> GAMEATPTPADLFSEDYLVDTLDGLTVDDQQAVLASLSFSKFLKHAKVRDWCAQAKIQPSMPALRMAYNYFLFSKVGEFIGSEDVCNFFVDRVFGGVRLLDVASVYAACSQMNAHQRHHICCLVERATSSQSLNPVWDALRDGIISSSKFHWAVKQQNTSKKIFSPWPITNNHFVAGPLAFGLRCEEVVKTLLATLLHPDETNCLDYGFMQSPQNGIFGVSLDFAANVKTDTEGRLQFDPNCKVYSIKCRFKYTFAKMECDPIYAAYQRLYEAPGKLALKDFFYSISKPAVEYVGLGKLPSESDYLVAYDQEWEACPRKKRKLTPLHNLIRECILHNSTTESDVYVLTDPQDTRGQISIKARFKANLFVNVRHSYFYQVLLQSSIVEEYIGLDSGIPRLGSPKYYIATGFFRKRGYQDPVNCTIGGDALDPHVEIPTLLIVTPVYFPRGAKHRLLHQAANFWSRSAKDTFPYIKWDFSYLSANVPHSP

Transition to the lytic phase coincides with the rapid degradation of ∼80% of all host mRNA transcripts in a process termed host shutoff (HSO) that is thought to promote immune evasion and enable viral co-option of the host replicative machinery. In the γ-herpesviridiae, HSO is initiated by the bifunctional alkaline exonuclease SOX that has been shown to possess exonucleolytic DNase and RNase activities. Owing to the presence of a PD-(D/E)XK sequence spanning two of seven conserved motifs shown to be essential for DNA turnover, KSHV SOX has been classified as a member of the type II restriction endonuclease-like superfamily confirmed by the crystal structures of the the related Epstein–Barr virus alkaline exonuclease BGLF5 (3) and apo form. More recent in vivo studies, however, indicate that SOX-mediated HSO is instead initiated by endonucleolytic ‘nicking’ of target transcripts followed by exonucleolytic degradation by the co-opted host scavenger exoribonuclease Xrn1 reminiscent of nonsense-mediated decay.

K2-31 was successfully co-crystallized with the SOX E244S catalytically inactive mutant (see Materials and Methods: Crystallization). Closer inspection revealed that K2-31 has a near continuous stem loop configuration, interrupted by the presence of a 7 nucleotide bulge (disordered in our structure) immediately 5΄ to the UGAAG motif. Interestingly, the protein-RNA contacts stabilising the complex are narrowly distributed with most restricted to the catalytic region and the K2-31 loop. In our structure, A20 and G21 at the apex are recognized by a series of hydrogen bonds involving Y373, R248 and F249. Further stabilization of K2-31 is derived from a stacking interaction between the adenine base of A20 and the aromatic side chain of F179 located in the bridge. In order to achieve this, F179 moves ∼5 Å (based on Cα-Cα distances) relative to its position in the DNA complex. Surprisingly, this alternative configuration of F179 and the N-terminal end of the bridge is stabilized by a disulphide bond between the sulphydryl groups of C183 and C247. Despite use of the inactivated E244S SOX mutant, the absence of density for A19 and lack of a phosphate group in close proximity to the essential catalytic carboxylate D221, is indicative of K2-31 having undergone cleavage over the duration of the crystallization experiment to produce a product complex. Inspection of the SOX-K2-31 structure reveals a complete absence of interactions between SOX and either the phophodiester backbone or bases of the UGAAG motif. Our mutagenesis studies have shown that while C247 has a minor role, F179 is essential for RNA but not DNA processing confirming the bridge as an important factor in substrate/product recognition where it directly functions in RNA binding as previously hypothesized.>MGWSDHDELSTDTTLHEEKFRIEPVPVHHQLDILKIAVSENYKTFASVGLDRSLVVWDLRQWCTKLVLSKEQMPRTLKAIALDPQGNYVSLFSKDTLFILNVESPSLMLQHSYHSKPNSKLNVFWMPGTHKDDEWKNFELVVVESSGEIQVFSLTIEIEGADIALVEKFQLSSPIIKSISIVSPTANRIASLTESGEVTVYSKKGPVWSPKILSQNKNYLTETKKDIYGIAMADILFLARDSGVDMIDLKNDELLHSFTLPPIKVNTFSVGV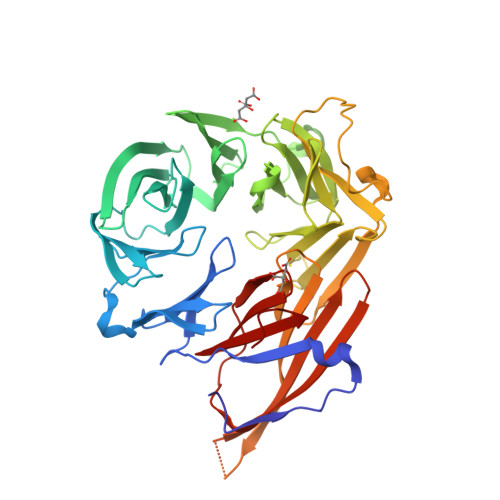SNSRFVNGQFRVSSISFCFTHAVTEKVLYYYYGNESNESYIILNKWDQQPNLVDVHDPDNSLASLTFDELQENIHEVEDASESVMSSDGLYIFGMRRKSSSGISPTADEKNEDNGFTLRNRKLRAGSNTHSGGETQVWEVWMYSQSEKKHRSKSLKMYNSLIIADPGPSLAVSDRCVAIVLGNYVALVGYGSEIFR[2x]>[2x]MHEQYQAPLPVNSPALPEPFYYLHNFRAVLAWIGERYADLLDDQERAFIAAFAELPEASQALLVRMVMRKGTLFREGKLAYAEIGDTRAAVQPLLALGWVDAQPTLELAQLFGLLKKDELSQLFRDHLGRANLRKDALLERLQPLFPEARRLAEWQADFAEPVYELRCMALCDRLRLMYFGNLWQDWSEFVLADLGIYRYESVEFSADSRGFRLRADVDAYLHLFDCRQRFDLGEPLEELLAGLPGEPYANPWLEGRRVKLLFQFAQ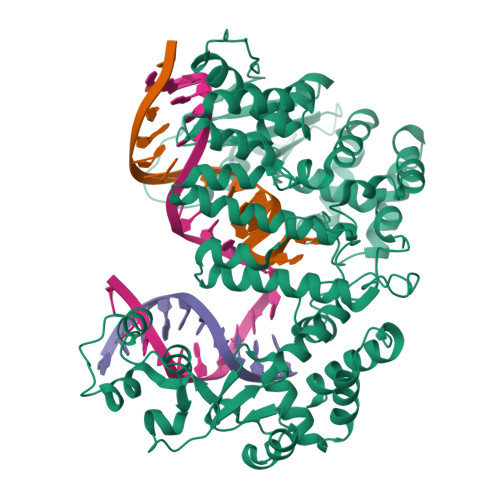HCEKQRDFDLAQRLYRQSSHPGARLRAIRSLERGERFAEAHALAREASCAPESDAERQGLARLLPRLQGKLGLPRQARAAAPEIDRLDLCLAFPSEPCSVEWAVREHLEEPGCAVHYVENGLINSLFGLLCWEAIFAAIPGAFFHPFHSAPADLHSADFRQRRAALFEACLGRLEDGSYRDAIRCRYRDKFGLQSPFVYWELLGEELLEQALDCLPAAHLRAWFERLLEDIPGNRAGLPDLIQFWPAQRRYRMVEVKGPGDRLQDNQLRWLQFCREREMPVAVCYVRWHVDD>[2x]MRAVNWNKKEDDFSLMFWKQNIAQFWTEEEIAVSSDKNTWVQLSKEEQIAYKRVLGGLTLLDTKQGGEGMPLVLVHLENLQAKSVLAFMGAMEEVHAKSYSHIFTTLATEEEIDEIFDWVDTHPLLEKKAGIITSYYRRLLKPEVTKKELYMAMVASVFLESYLFYSGFFYPLYLAGQGKLTASGEIINLIIRDESIHGVFVGILAQQIFAELSAEDQQEVQKETQELLMELYEIEMAYTEEIYTSIGLVEDVNRFVRYNANKGLMNLGLEPKFEEEEINPIVLNGLRTDTKNHDFFSVKGNGYVKATNVEKLSDDDFVFNF

Ribonucleotide reductase (RNR) is a key enzyme in all domains of life, utilizing radical chemistry for the synthesis of deoxyribonucleotides by substitution of the 2′ OH-group of a ribose 5′phosphate with a hydrogen. The strictly aerobic class I RNRs are comprised of two homodimeric subunits: a large catalytic subunit R1, where ribonucleotide reduction takes place, and a small radical-generating subunit R2. R2a proteins utilize an oxygen-activated di-ferrous metal site to generate a stable FeIII/FeIII-tyrosyl radical (Y·) cofactor, whereas R2b proteins generate a MnIII/MnIII-Y·. R2c proteins generate a MnIV/FeIII cofactor and the recently discovered class R2d—a MnIV/MnIII cofactor. These dimetal centers reside in a ferritin-like scaffold, and are coordinated by two histidine residues and four carboxylate ligands.

Here we show that the class Ib ribonucleotide reductase R2 protein from Bacillus anthracis spontaneously assembles a Mn/Mn cofactor in vitro, under both aerobic and anoxic conditions, when the metal-free protein is subjected to incubation with MnII and FeII in equal concentrations. To study metal selectivity and cofactor assembly from a mixed MnII and FeII pool in the presence and absence of O2, in the present study we describe apoprotein crystal soaking experiments, subjecting apo BaR2b to a large excess of both MnII and FeII in aerobic and reducing anoxic conditions (in presence of 30 mM sodium dithionite). Site-specific metal quantification by X-ray anomalous dispersion on WT BaR2b revealed that the two sites of the metal center predominantly bind Mn irrespective of the presence or absence of O2 in the experimental setup. Unlike R2lox and R2c, wild-type BaR2b is able to select Mn over Fe in both binding sites. The capability to exclude Fe appears central for a protein requiring a di-Mn cofactor for function. If Mn binds in both positions, neither the wild-type nor the L61G reacts with O2.>GPEFEAAACKKYMSKLRTIVAAQSRFLSTYDGAENLCLEDIYTENTLEVRTEVGMAGPLHKSPAALGLEELFSPNGHLNEDADTVLVVGEAGSGKSTLLQQVHLLWATGQDFQEFLFVFPFSCRQLQCVARPLSVMTLLFEHCCWPDVGQQDVFQFLLDHPDRILLTFDGFDEFKFKFTDHERHCSPTDPTSVQTLLFNLLQGNLLKNARKVLTSRPDAVSAFLRKYVRTEFNLKGFSEEGIELYLRKCHREPGVADRLIHLLQTTSALHGLCHLPVFSWMVSKCHQELLLQDGGSPKTTTDMYLLILQHFLRHASLPDSASQGLGPSLLQGRLPTLLRLGQLALWGLGMCCYVFSAQQLQAAQVDPDDISLGFLVQAQGVVPGSTAPLEFLHITFQCFLAAFYLVLSTDVPTASLRYLFNCRRPGSSPLSRLLPRLCVQGSEHKESTVAALLQKTEPHNLQITAAFLAGLLSREHRDLLAACQASERSLLRRRACARWCLARSLHKHFRSIPPAVPGEAKSMHAMPGFLWLIRSLYEMQEERLAQEAVRGLNVEHLKLTFCGVGPAECAALAFVLRHLRRPVALQLDHNSVGDIGVEQLLPCLGACKALYLRDNNISDRGICKLIEHALHCEQLQKLALFNNKLTDGCAHSVAQLLACKQNFLALRLGNNHITAEGAQVLAEGLRDNSSLQFLGFWGNKVGDKGAQALAEALSDHQSLKWLSLVGNNIGSVGAQALASMLEKNVALEELCLEENHLQDAGVCSLAEGLKRNSSLKVLKLSNNCITFVGAEALLQALASNDTILEVWLRGNPFSPEEMEALSHRDSRLLL[2x]

NOD2, also known as NLRC2 or CARD15, belongs to the NLRC subfamily of NLRs. NOD2 possesses two tandem CARDs that function as an effector domain and is activated by muramyl dipeptide (MDP), a bacterial cell wall fragment9101112. On activation by MDP, NOD2 is believed to undergo self-oligomerization via the central NOD domain, providing a scaffold for recruiting RIPK2 (receptor-interacting serine–threonine kinase 2) through CARD–CARD interactions. Here, we determined the crystal structure of the inactive ADP-bound form of NOD2, and revealed that ADP-bound NOD2 is maintained in an auto-inhibited/closed form through ADP-mediated and inner domain interactions of the NOD domain.

We also generated a construct in which we deleted the loop regions encoded in residues 245–251 and 626–635, in addition to the removal of the CARD (OcNOD2ΔCARDΔloop), because residues 245–251 are not conserved in zebrafish NOD2 and residues 626–635 are susceptible to proteolytic cleavage during purification. We crystallized OcNOD2ΔCARDΔloop in two forms (form 1 and form 2) under different crystallization conditions and determined the crystal structures at 2.3 Å (form 1) and 3.3 Å (form 2) resolutions. The asymmetric unit of the form 1 and form 2 crystals contained one and two NOD2 molecules, respectively. The structures of the NOD2 molecules in these crystals were essentially the same, with root mean squared deviations (r.m.s.d.) between 0.4 and 1.1 Å. Since we observed no noticeable differences among these three crystal structures, we refer, hereafter, to the structure of OcNOD2ΔCARDΔloop in the form 2 crystal unless otherwise noted. The crystal structure showed that ADP-bound NOD2 folded into a hook-shaped structure with dimensions of ∼70 × 80 × 40 Å, consisting of a NOD domain (residues 195–744) and a LRR domain (residues 745–1,020). The NOD domain can be further divided into the nucleotide-binding domain (NBD, residues 195–425), helical domain 1 (HD1, residues 426–485), the winged-helix domain (WHD, residues 486–602) and helical domain 2 (HD2, residues 603–743), similar to other NOD domains with known structures. The LRR domain of NOD2 consisted of ten LRR units and formed a typical horseshoe-like structure in a single curvature, with α-helices forming the convex surface and β-strands in the concave faces. ADP embedded at the centre of the NOD domain bridged the NBD and HD1, and bound to the WHD, allowing the subdomains to be closely packed. As the resulting structure of NOD2 folded into a compact tertiary arrangement, we concluded that the crystal structure of OcNOD2ΔCARD is that of a closed and inactive conformation.>MNSNVENLPPHIIRLVYKEVTTLTADPPDGIKVFPNEEDLTDLQVTIEGPEGTPYAGGLFRMKLLLGKDFPASPP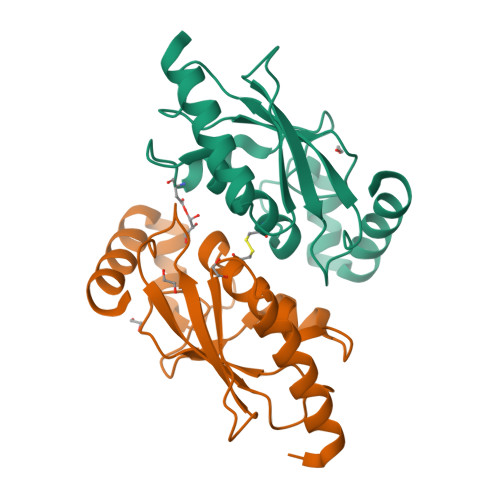KGYFLTKIFHPNVGANGEICVNVLKRDWTAELGIRHVLETIKCLLIHPNPESALNEEAGRLLLENYEEYAARARLLTEIHG[2x]3-(naphthalen-1-ylmethyl)-1-(piperidin-4-ylmethyl)-1H-pyrazolo[3,4-d]pyrimidin-4-amine | C22 H24 N6 | 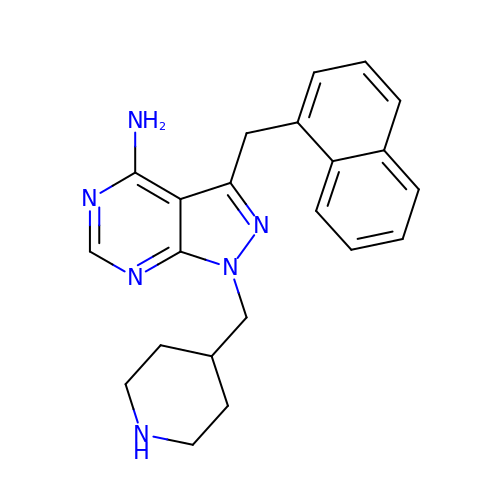MMRLNUFECMEMSQ-UHFFFAOYSA-N>MSFIRTFYGDIAPEQLGFTYSHEHIVCVPAYWQERDADDLLLDDKEKSQLDVQDFADLGGKTIVDATAVDYGRRVLDVAQISKETGIQIVGTAGFNKSFLWDGKIKPELKPIIGDFETYYEWIENTTTDKLTEFVVNEVENGLEGTPYKAGQVKFGTGYNMITPLEEKTIRAVARAHHETKAPIHSHTEAGTMALEQIEILKQENIPLEYLSIGHMDRNLDPYYHKQVAKTGAFMSFDGIAKIKYAPESARIAAILYLVSEGFEDQILVSGDTARKTYYKHYGHGPGLEYIAKKWVPRFIDEANEKGFDGEKLVKKFFVDNPARCFTFKK[6x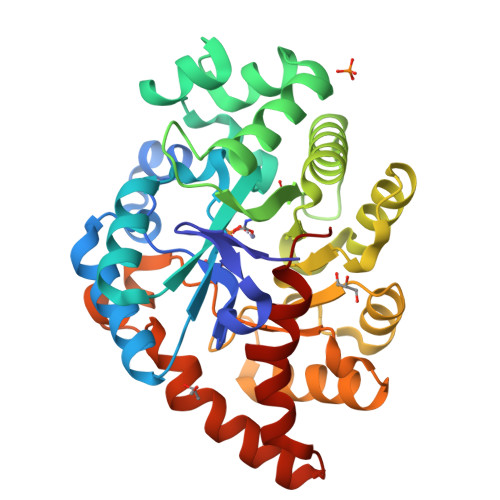]>NAMIIRPEQHWFLRLFDWHGSVLSKIIFRLLLNVLMSIIAIISYQWYEQLGIHLTVAPFSLLGIAIAIFLGFRNSASYSRFVEARNLWGTVLIAERTLVRQLRNILPAEHDAHRRIVSYLVAFSWSLKHQLRKTDPTADLRRLLPEERVTEILASSMPTNRILLLAGNEIGQLREAGKLSDITYGLMDNKLDELAHVLGGCERLATTPVPFAYTLILQRTVYLFCTLLPFALVGDLHYMTPFVSVFISYTFLSFDSLAEELEDPFGTAANDLPLNAMCNTIERNLLDMTGQHPLPE[5x]

Human bestrophin1 (hBest1) is a Ca2+-activated Cl− channel essential for Cl− transport in retinal pigment epithelium (RPE). Although the structure of hBest1 is still unsolved, two Best1 homolog structures, one from bacteria Klebsiella pneumoniae (KpBest) and the other from chicken (cBest1), have been previously reported. Overall, the channel is a pentameric assembly with a single ion-conducting pathway, which varies in diameter along its length and is constrained at two narrow points: a “neck” contributed by three residues (I62/I66/F70 in KpBest and I76/F80/F84 in hBest1/cBest1) on a transmembrane helix, and an “aperture” formed by a single residue (I180 in KpBest1, I205 in hBest1, and V205 in cBest1) on a cytosolic helix. Here, by electrophysiological and structural analyses, we show that the neck and aperture in hBest1 are both indispensable Ca2+-dependent gates, and their dysregulated opening by rationally designed or patient-derived mutations causes Ca2+-independent leak and elevates Ca2+-dependent channel activity.

The Y236A, Y236C, and W287F mutants all conducted Ca2+-dependent Cl− currents significantly bigger than those from WT hBest1 under the same conditions, indicating gain-of-function phenotypes. Moreover, the Y236C and W287F mutants retained the CH3SO3− to Cl− relative permeability but not the trans-promotive effect of CH3SO3−, functionally resembling hBest1 3A, rather than hBest1 I205A. As the cBest1 3A mutant structure shows a constantly unconstrained neck, the gain-of-function in Y236A, Y236C, and W287F is likely a result of enhanced open probability of the neck. Moreover, consistent with our conclusion that hBest1 W287F is a gain-of-function mutation with increased open probability of the neck, a cBest1 W287F mutant structure shows a constantly opened neck. To understand the structural bases of these mutants, we solved the structures of KpBest Y211A, W252A, and W252F at 2.6, 2.5, and 3.1 Å (equivalent to hBest1 Y236A, W287A, and W287F), respectively. Consistent with the functional results, no structural change was found at the aperture. Although the structure at the neck region was surprisingly unaltered, possibly due to the molecular packing effect in the crystal or the presence of Zn2+ in the crystallization solution which might stabilize the channel in a closed state, all three KpBest mutants displayed conformational changes on P208, Y211, and W252 (equivalent to P233, Y236, and W287 in hBest1, respectively), reaffirming the mutual influence between these three residues. Therefore, W287 is an extremely sensitive “switch” of the neck.N-{2-[4-methoxy-3-(2-phenylethoxy)phenyl]ethyl}-N-propylpropan-1-amine 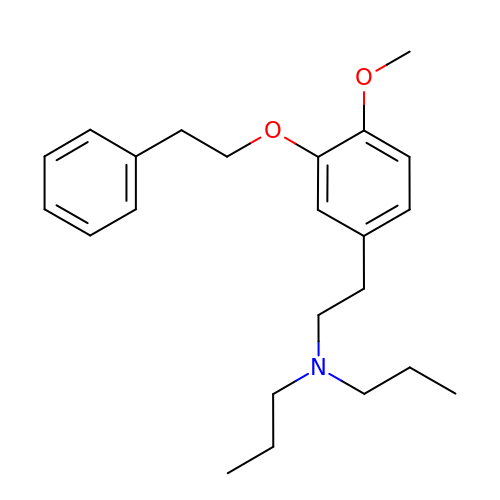| C23 H33 N O2 | YBLIQJGXRLZBCZ-UHFFFAOYSA-N>MNTVSPAKKKVIIIGAGIAGLKAASTLHQNGIQDCLVLEARDRVGGRLQTVTGYQGRKYDIGASWHHDTLTNPLFLEEAQLSLNDGRTRFVFDDDNFIYIDEERGRVDHDKELLLEIVDN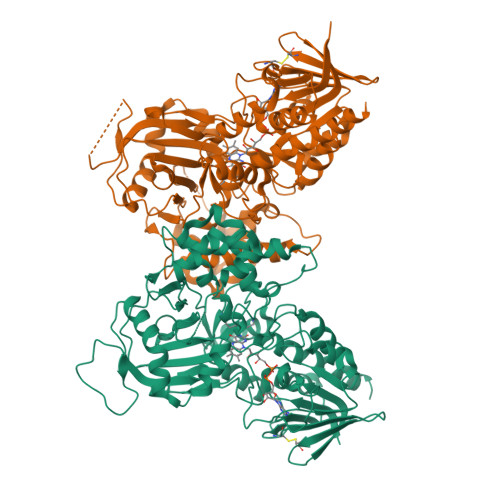EMSKFAELEFHQHLGVSDCSFFQLVMKYLLQRRQFLTNDQIRYLPQLCRYLELWHGLDWKLLSAKDTYFGHQGRNAFALNYDSVVQRIAQSFPQNWLKLSCEVKSITREPSKNVTVNCEDGTVYNADYVIITVPQSVLNLSVQPEKNLRGRIEFQPPLKPVIQDAFDKIHFGALGKVIFEFEECCWSNESSKIVTLANSTNEFVEIVRNAENLDELDSMLEREDSQKHTSVTCWSQPLFFVNLSKSTGVASFMMLMQAPLTNHIESIREDKERLFSFFQPVLNKIMKCLDSEDVIDGMRPIENIANANKPVLRNIIVSNWTRDPYSRGAYSACFPGDDPVDMVVAMSNGQDSRIRFAGEHTIMDGAGCAYGAWESGRREATRISDLLKLEHHHHHH[2x]In this work we report on the sat encoded dissimilatory ATP sulfurylase from the sulfur-oxidizing purple sulfur bacterium Allochromatium vinosum. The genes cysDN (Alvin_2448 and Alvin_2449) encode for ATPS in an unusual sulfate assimilation pathway and the gene sat (Alvin_1118) for an ATPS involved in the dissimilatory sulfur oxidation pathway, respectively. Dissimilatory sulfur-oxidizing ATPS was found to exist as a homodimer. We produced the purple bacterial sat-encoded ATP sulfurylase as a recombinant protein in E. coli, determined crucial kinetic parameters and obtained a crystal structure in an open state with a ligand-free active site.

The asymmetric unit contains one homodimer of ATPS with rms differences between the monomers being 1.4 Å. No significant differences were detectable between them except for a rigid-body movement of the C-terminal relative to the other domains in the range of 4 Å and of segment 233∶239 which contacts the C-terminal domain. The N-terminal domain I (residues 1–172) is basically built up of a β barrel with five antiparallel strands surrounded by α-helices, the catalytic domain II (residues 173–331) of a typical Rossmann-like α/β structure and the small C-terminal domain III (residues 332–396) of a small three-strand β-sheet and two α-helices. The structure of ATPS of A. vinosum was determined without any ligand in the active site. Two MES (2N-morpholino-ethansulfonic acid) molecules (present in the crystallization solution) could be, however, identified close to the monomer-monomer interface far away from the active site. In the A. vinosum ATPS structure the active site is only occupied by water molecules; more than ten of them are visible in the electron density map. The catalytic process starts by binding APS into the empty active site groove best expressed by the A. vinosum ATPS structure present in an open form. The conserved GxxKxxD loop after strand 9 (224∶230) is in an “up” position and highly mobile in the open A. vinosum and “Candidatus E. persephone” ATPS. The open form of the C-terminal domain of ATPS of A. vinosum interferes with the pyrophosphate binding site which is created upon APS binding in the closed form in front of the N-terminal side of helix 12 (361∶370). First, in A. vinosum ATPS the GxxKxxD loop is in direct contact to the partner monomer.

>[2x]MIKPVGSDELRPRFVYDPEQHHRLSSEAESLPSVIVSSQAAGNAVMLGAGYFSPLDGFMNLADALSSAQSMTLTDGRFFPVPLLCLLESADAIAGATRIALRDPNVEGNPVLAVMDVTAVEQVSDAQMALMTEQVYGTSDPKHPGVETFNSQGRTAISGPIQVLNFSYFQTDFPDTFRTAVEIRHEIQERGWQKIVAFQTRNPMHRAHEELCKMAMEAVEADGVVIHMLLGQLKPGDIPAPVRDAAIRTMAELYFPPNTVMVTGYGFDMLYAGPREAVLHAYFRQNMGATHFIIGRDHAGVGDYYGPFDAQTIFDDAVPTDVLAIEIFRADNTAYSKKLGRVVMMRDAPDHTPDDFIQLSGTRVREMLGQGEAPPPEFSRPEVAQILMDYYRSLPQS(Z)-3-[3,4-bis(oxidanyl)phenyl]-2-oxidanyl-1-[2,4,6-tris(oxidanyl)phenyl]prop-2-en-1-one | C15 H12 O7 | 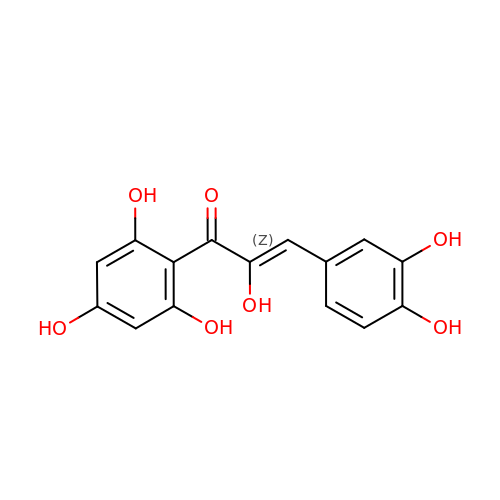CUYYQQQQHCDPCX-PQMHYQBVSA-N2-(pyridin-3-ylmethoxy)aniline | C12 H12 N2 O | 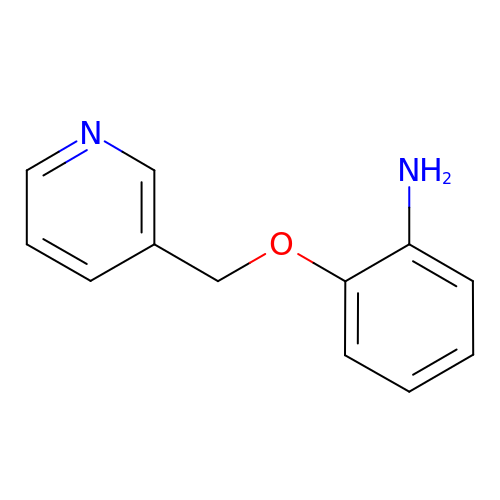NISBBHHUQZRGQA-UHFFFAOYSA-N Human LLT1 is a C-type lectin-like ligand of NKR-P1 (CD161, gene KLRB1), a C-type lectin-like receptor of natural killer cells. Similarly to mouse Clr-g, human LLT1 is a type II transmembrane glycoprotein which consists of an N-terminal cytoplasmic chain, transmembrane and stalk regions and a C-terminal CTL domain with two predicted N-linked glycosylation sites. The engagement of NKR-P1 on the NK cell with LLT1 on the target cell inhibits NK cell cytotoxicity and IFNγ production and contributes to NK self-tolerance in a similar way to the orthologous rodent NKR-P1B–Clr-b receptor–ligand pair. In this study, we present several structures of LLT1 under various conditions: monomeric (LLT1_mono), dimeric deglycosylated after the first N-acetyl­glucosamine unit (LLT1_D1 and LLT1_D2) and dimeric (packed into hexamers) with homogeneous GlcNAc2Man5 glycosylation (LLT1_glyco).

The dimeric form follows the classical dimerization mode of human CD69. The protein used to obtain the LLT1_glyco structure contained homogeneous GlcNAc2Man5 glycosylation, while the protein used to obtain the LLT1_mono, LLT1_D1 and LLT1_D2 structures was deglycosylated beyond the first GlcNAc. LLT1_glyco, LLT1_D1 and LLT1_D2 share essentially the same structure at the level of the dimer; however, they differ slightly in the mutual orientation of the monomers within a dimer. In contrast, it is 173.7° for LLT1_D1 and 177.7° for LLT1_D2, both of which crystallized in space group P212121 with one dimer in the asymmetric unit. The dimeric interface in all three LLT1 dimers is based on a hydrophobic core formed by phenyl rings, analogous to that observed in similar CTL dimers: Phe121, Tyr125, Phe89, Phe87 and Phe82. Additionally, there is an interaction formed by π-stacking of arginine residue Arg124 of both chains, and a pair of His190 residues forms a partial stacking interaction in the termini region (the part of the CTL domain oriented towards the cell membrane). There are six common hydrogen bonds that connect the monomers in all three dimers: AGly81 N–BGly81 O, AArg124 N∊–BTyr125 O, AArg124 Nη1–BLys126 O and the three analogous hydrogen bonds with exchanged chains. Additionally, there are some hydrogen bonds specific to individual cases: one additional hydrogen bond in the dimeric interface of LLT1_glyco, two hydrogen bonds in LLT1_D2 and six in LLT1_D1. As an example, residue His190, localized near the C-terminus in the dimerization interface, is charged at low pH and destabilizes this part of the interface. It is apparent from the structures that His190 is neutral in LLT1_D1 and LLT1_D2 (pH 7.0) and is close to His190 (3.1 and 3.3 Å) from the opposite chain, participating in a partial stacking inter­action.

>ITGQAACPESWIGFQRKCFYFSDDTKNWTSSQRFCDSQDADLAQVESFQELNFLLRYKGPSDHWIGLSREQGQPWKWINGTEWTRQFPILGAGECAYLNDKGASSARCYTERKWICSKSDIHVGTKHHHHHHHHG[2x]>[2x]MAKKKKKKSFNTTRPTDPPVYPVTVPFLGHIVQFGKNPLEFMQRCKRDLKSGVFTISIGGQRVTIVGDPHEHSRFFSPRNEILSPREVYTIMTPVFGEGVAYAAPYPRMREQLNFLAEELTIAKFQNFVPAIQHEVRKFMAENWKEDEGVINLLEDCGAMIINTACQCLFGEDLRKRLNARHFAQLLSKMESSLIPAAVFMPWLLRLPLPQSARCREARAELQKILGEIIVAREKEEASKDNN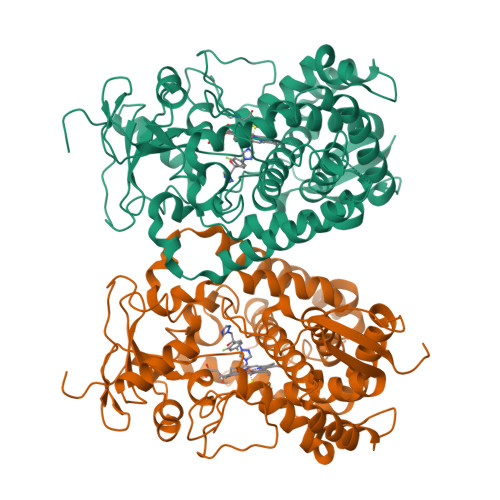TSDLLGGLLKAVYRDGTRMSLHEVCGMIVAAMFAGQHTSTITTSWSMLHLMHPKNKKWLDKLHKEIDEFPAQLNYDNVMDEMPFAERCVRESIRRDPPLLMVMRMVKAEVKVGSYVVPKGDIIACSPLLSHHDEEAFPNPRLWDPERDEKVDGAFIGFGAGVHKCIGQKFALLQVKTILATAFREYDFQLLRDEVPDPDYHTMVVGPTLNQCLVKYTRKKKLPSHHHHHH> EVT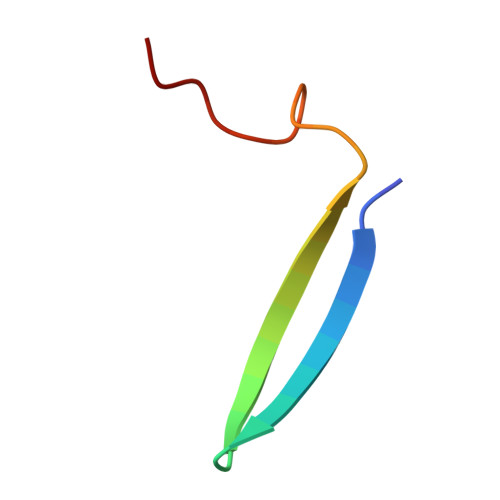VTDITANSITVTFREAQAAEGFFRDRS5-{[(2S)-2-aminopropyl]amino}-3-(1H-indol-2-yl)pyrazine-2-carboxamide 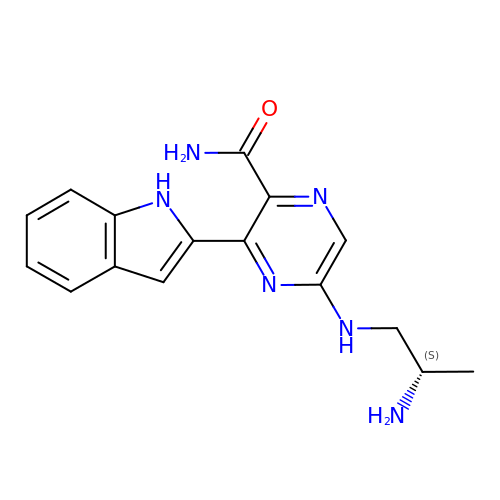| C16 H18 N6 O | NYYIGJQYEWZYJP-VIFPVBQESA-N5'-amino-5'-deoxyadenosine 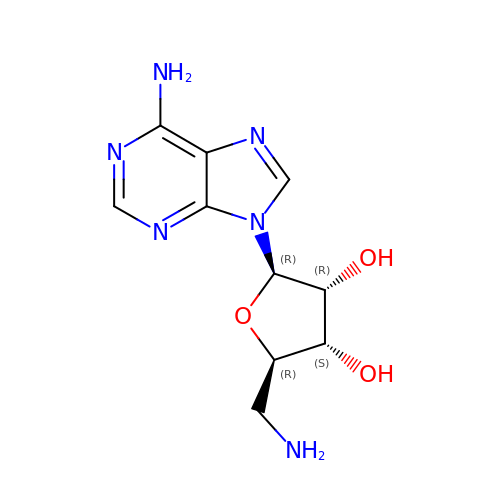| C10 H14 N6 O3 | GVSGUDGNTHCZHI-KQYNXXCUSA-N Filamentous bacteriophages package their circular, single stranded DNA genome with the major coat protein pVIII and the minor coat proteins pIII, pVII, pVI, and pIX. Here, we report the cryo-EM structure of a ~500 Å long bacteriophage M13 mini variant. The distal ends of the mini phage are sealed by two cap-like complexes composed of the minor coat proteins. We further performed local refinements of the mini phage by dividing the particle into the top, middle and bottom three segments.

Our reconstruction of the bottom cap reveals a pencil-tip-like structure, where five pIIIs and five pVIs form a sharp cap enwrapping the pVIII cylinder. Both pIII and pVI have a hook-like structure with two long helices (helixLN and helixLC), located at the N- and C-termini of the structures, respectively. In addition to these two long helices, pIII has a short helix at the N-terminus, and two short helices (middle short helices) and a long loop situated in between the two long helices, while pVI has only a short helix in between the two long helices. The N-terminal short helices of pIIIs assemble into a helix barrel, maintained by hydrophobic interactions and hydrogen bonds. The helixLNs of pIIIs and pVIs tighten at the bottom of the cap and alternately distribute with intervals, forming a sharp-tip like helix barrel. In this structure, the helixLNs from pIIIs are located at the outer positions while the helixLNs of pVIs occupy the inner positions. In the sharp-tip like helix barrel, the outer surface of pVI is predominantly hydrophobic but contains two positively charged rings that are formed by R12, K30, and K31 in the helixLN. However, the helixLN of pIII is rich in negatively charged residues, which are in close proximity to the positively charged regions of pVI and shield the hydrophobic surface of pVI. The middle part of the pIII long loop forms a β-hairpin structure, rich in aromatic residues, which inserts into a pocket formed by residues of three pVIII helices from layers 21, 22, and 23. However, in comparison to the interactions with pVIII at the same location, the interactions with pIII are more extensive, indicating that pIII may be able to effectively compete with pVIII for binding the pocket.

>AETVESCLAKPHTENSFTNVWKDDKTLDRYANYEGCLWNATGVVVCTGDETQCYGTWVPIGLAIPENEGGGSEGGGSEGGGSEGGGTKPPEYGDTPIPGYTYINPLDGTYPPGTEQNPANPNPSLEESQPLNTFMFQNNRFRNRQGALTVYTGTVTQGTDPVKTYYQYTPVSSKAMYDAYWNGKFRDCAFHSGFNEDPFVCEYQGQSSDLPQPPVNAGGGSGGGSGGGSEGGGSEGGGSEGGGSEGGGSGGGSGSGDFDYEKMANANKGAMTENADENALQSDAKGKLDSVATDYGAAIDGFIGDVSGLANGNGATGDFAGSNSQMAQVGDGDNSPLMNNFRQYLPSLPQSVECRPFVFGAGKPYEFSIDCDKINLFRGVFAFLLYVATFMYVFSTFANILRNKES[5x];>[15x]MKKSLVLKASVAVATLVPMLSFAAEGDDPAKAAFNSLQASATEYIGYAWAMVVVIVGATIGIKLFKKFTSKAS;>MPVLLGIPLLLRFLGFLLVTLFGYLLTFLKKGFGKIAIAISLFLALIIGLNSILVGYLSDISAQLPSDFVQGVQLILPSNALPCFYVILSVKAAIFIFDVKQKIVSYLDWDK[5x]> 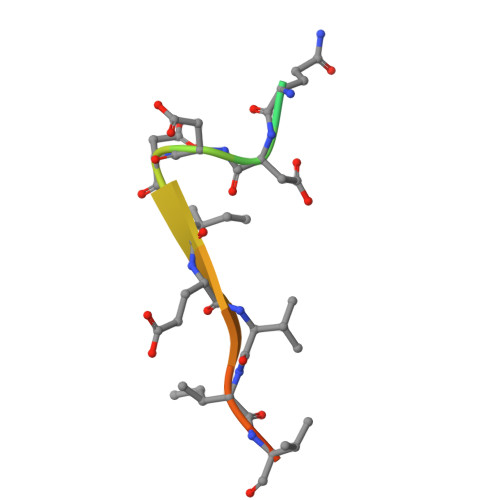GPGSEQDDDIEVIVDET>[3x]MTAESPTIRLERYSERHVEGLTALYNDPAVARQVLQMPYQSVEQRRKRLHDSADDDRLLILVALHQGDVIGSASLEQHPR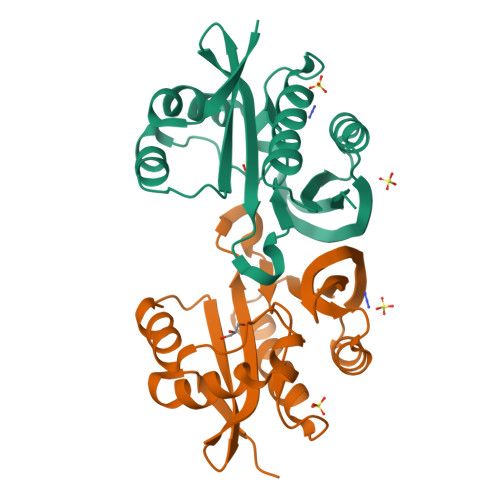IRRSHSGSIGMGVAVAWQGKGVGSRLLGELLDIADNWMNLRRVELTVYTDNAPALALYRKFGFETEGEMRDYAVRDGRFVDVYSMARLRRVEGRVGE> QLK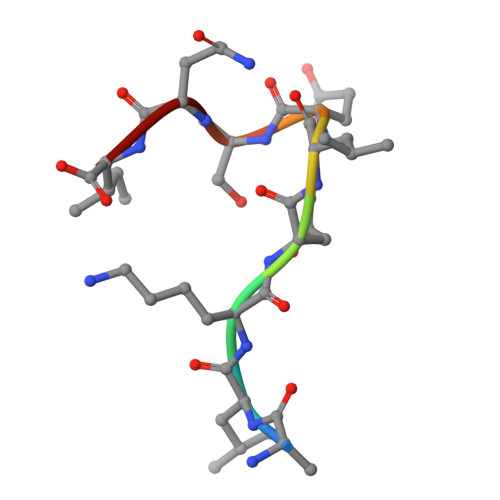DLESQI> DEEQVFHFYWLDAYEDQYNQPGVVFLFGKVWIESAETHVSCCVMVKNIERTLYFLPREMKIDLNTGKETGTPISMKDVYEEFDEKIATKYKIMKFKSKPVEKNYAFEIPDVPEKSEYLEVKYSAEMPQLPQDLKGETFSHVFGTNTSSLELFLMNRKIKGPCWLEVKSPQLLNQPVSWCKAEAMALKPDLVNVIKDVSPPPLVVMAFSMKTMQNAKNHQNEIIAMAALVHHSFALDKAAPKPPFQSHFCVVSKPKDCIFPYAFKEVIEKKNVKVEVAATERTLLGFFLAKVHKIDPDIIVGHNIYGFELEVLLQRINVCKAPHWSKIGRLKRSNMPKLGGRSGFGERNATCGRMICDVEISAKELIRCKSYHLSELVQQILKTERVVIPMENIQNMYSESSQLLYLLEHTWKDAKFILQIMCELNVLPLALQITNIAGNIMSRTLMGGRSERNEFLLLHAFYENNYIVPDKQIFRKPQQKLGDEDEEIDGDTNKYKKGRKKAAYAGGLVLDPKVGFYDKFILLLDFNSLYPSIIQEFNICFTTVQRVASEAQKVTEDGEQEQIPELPDPSLEMGILPREIRKLVERRKQVKQLMKQQDLNPDLILQYDIRQKALKLTANSMYGCLGFSYSRFYAKPLAALVTYKGREILMHTKEMVQKMNLEVIYGDTDSIMINTNSTNLEEVFKLGNKVKSEVNKLYKLLEIDIDGVFKSLLLLKKKKYAALVVEPTSDGNYVTKQELKGLDIVRRDWCDLAKDTGNFVIGQILSDQSRDTIVENIQKRLIEIGENVLNGSVPVSQFEINKALTKDPQDYPDKKSLPHVHVA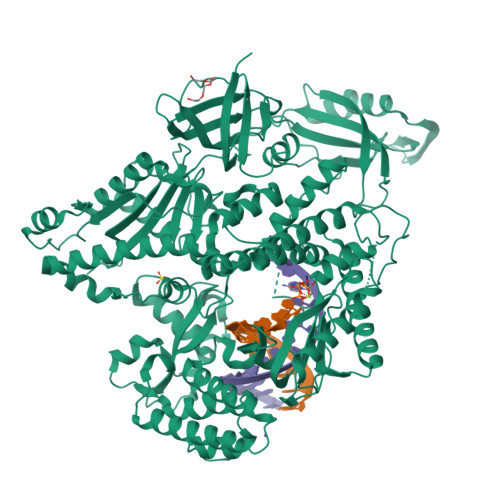LWINSQGGRKVKAGDTVSYVICQDGSNLTASQRAYAPEQLQKQDNLTIDTQYYLAQQIHPVVARICEPIDGIDAVLIATWLGLDPTQFRVHHYHKDEEN> PGTVDKKMVEKCWKLMDKVVRLCQNPKLALKNSPPYILDLLPDTYQHLRTILSRYEGKMETLGENEYFRVFMENLMKKTKQTISLFKEGKERMYEENSQPRRNLTKLSLIFSHMLAELKGI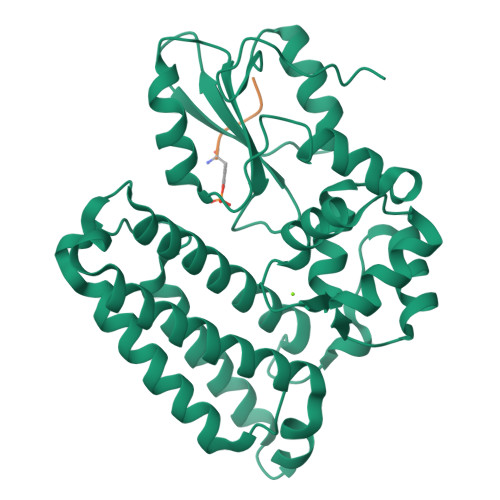FPSGLFQGDTFRITKADAAEFWRKAFGEKTIVPWKSFRQALHEVHPISSGLEAMALKSTIDLTCNDYISVFEFDIFTRLFQPWSSLLRNWNSLAVTHPGYMAFLTYDEVKARLQKFIHKPGSYIFRLSCTRLGQWAIGYVTADGNILQTIPHNKPLFQALIDGFREGFYLFPDGRNQNPDLTG>MLKFMLDTNICIFTIKNKPASVRERFNLNQGKMCISSVTLMELIYGAEKSQMPERNLAVIEGFVSRIDVLDYDAAAATHTGQIRAELARQGRPVGPFDQMIAGHARSRGLIIVTNNTREFERVGGLRTEDWS[4x];>[4x]MHHHHHHETTVFLSNRSQAVRLPKAVALPENVKRVEVIAVGRTRIITPAGETWDEWF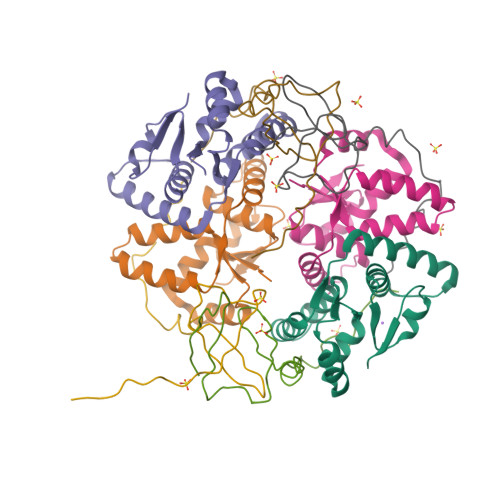DGHSVSTDFMDNREQPGMQERESF> ACDYTCGSNCYSSSDVSTAQAAGYKLHEDGETVG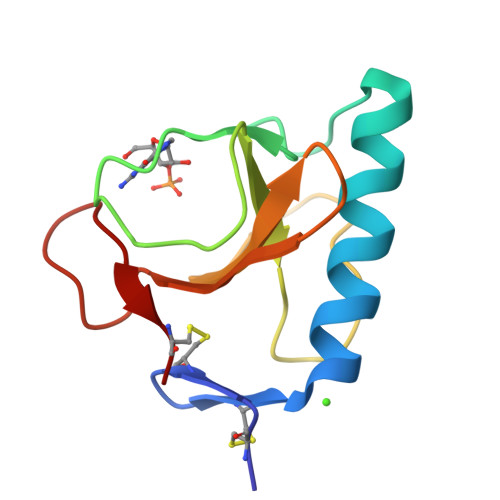SNSYPAKYNNYEGFDFSVSSPYYEWPILSSGDVYSGGSPGADRVVFNENNQLAGVITHTGASGNNFVECT> GSAAASPAWMPAYACQRPTPLTHHNTGLSEALEILAEAAGFEGSEGRLLTFCRAASVLKALPSPVTTLSQLQGLPHFGEHSSRVVQELLEHGVCEEVERVRRSERYQTMKLFTQIFGVGVKTADRWYREGLRTLDDLREQPQKLTQQQKAGLQHHQDLSTPVLRSDVDALQQVVEEAVGQALPGATVTLTGGFRRGKLQGADVDFLITHPKEGQEAGLLPRVMCRLQDQGLILYHQHQHSCCESPTRLAQQSHMDAFERSFCIFRLP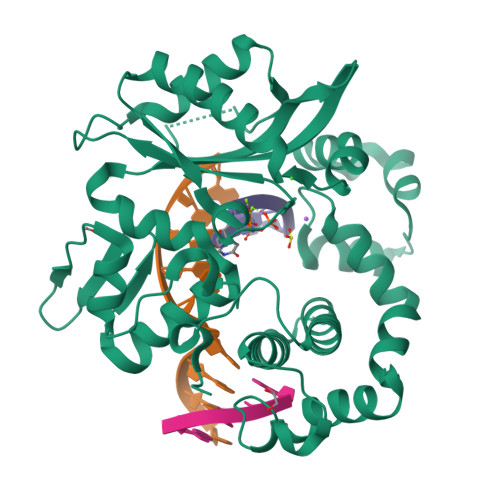QPGSWKAVRVDLVVAPVSQFPFALLGWTGSKLFQRELRRFSRKEKGLWLNSHGLFDPEQKTFFQAASEEDIFRHLGLEYLPPEQRNA> MEDQLSRRLAALR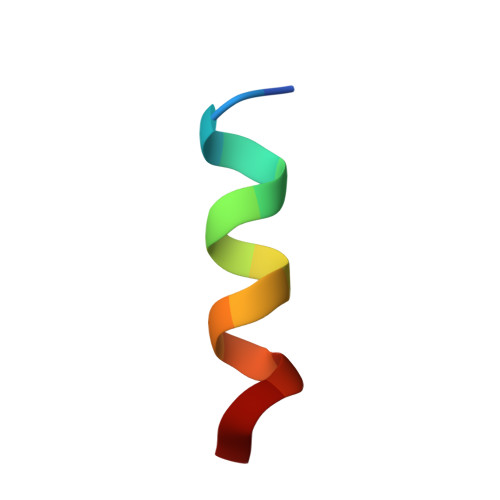N> HHHHHHMVRAIDEDCSQYEPIPGSQKAALGYNILTQEDAQSVYDASYYGGQCETVYNGEWRELRYDSTCERLYYGDDEKYFRKPYNFLKYHFEALADTGISSEFYDNANDLLSKVKKDKSDSFGVTIGIGPAGSPLLVGVGVSHSQDTSFLNELNKYNEKKFIFTRIFTKVQTAHFKMRKDDIMLDEGMLQSLMELPDQYNYGMYAKFINDYGTHYITSGSMGGIYEYILVIDKAKMESLGITSRDITTCFGGSLGIQYEDKINVGGGLSGDHCKKFGGGKTERARKAMAVEDIISRVRGGSSGWSGGLAQNRSTITYRSWGRSLKYNPVVIDFEMQPIHEVLRHTSLGPLEAKRQ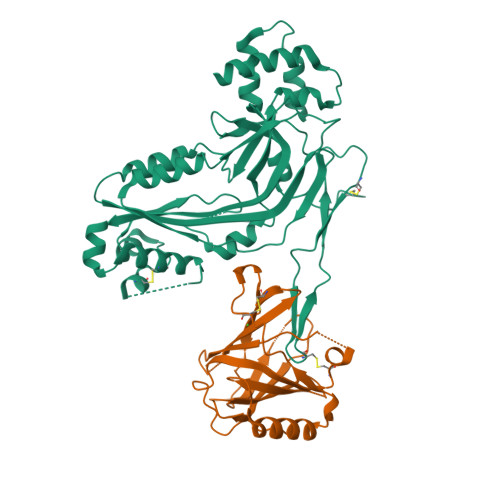NLRRALDQYLM;> MAQKPQRPRRPASPISTIQPKANFDAQQFAGTWLLVAVGSACRFLQEQGHRAEATTLHVAPQGTAMAVSTFRKLDGICWQVRQLYGDTGVLGRFLLQARDARGAVHVVVAETDYQSFAVLYLERAGQLSVKLYARSLPVSDSVLSGFEQRVQEAHLTEDQIFYFPKYGFCEAADQFHVLDEVRR> VDYAPAQAQIVHAGQACVVKEDNISERVYTIREGDTLMLQCLVTGHPRPQVRWTKTA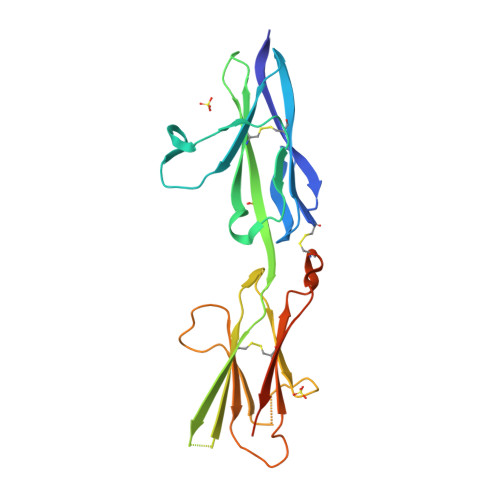GSASDKFQETSVFNETLRIERIARTQGGRYYCKAENGVGVPAIKSIRVDVQYLDEPMLTVHQTVSDVRGNFYQEKTVFLRCTVNSNPPARFIWKRGSDTLSHSQDNGVDIYEPLYTQGETKVLKLKNLRPQDYASYTCQVSVRNVCGIPDKAITFRLTNTTGSASTSHHHHHH> L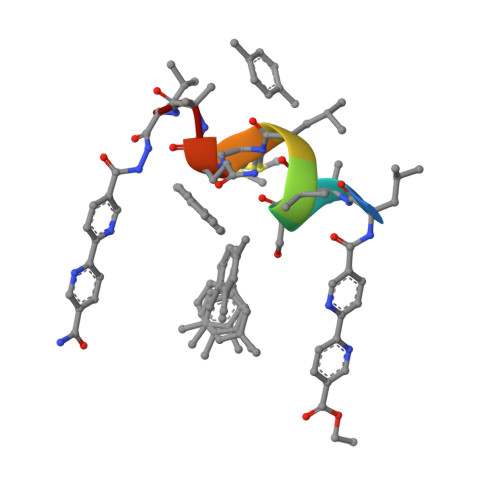ASALMQAL>MAIDEIKSRGYLLVGLSADFPPFEFVDENGNIVGFDVDLAKEIARRLGVELKIVDMTFDGLIPSLLTKKIDVIISGMTITEERKKVVAFSDPYFDAGGGG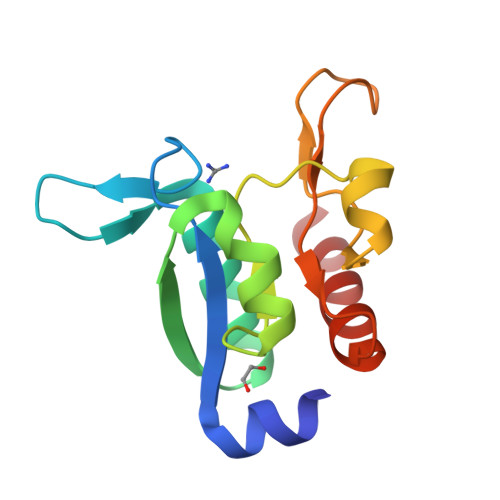SGEQYGIAVRKEDTDLLEFINSVLRELK[2x]> MDE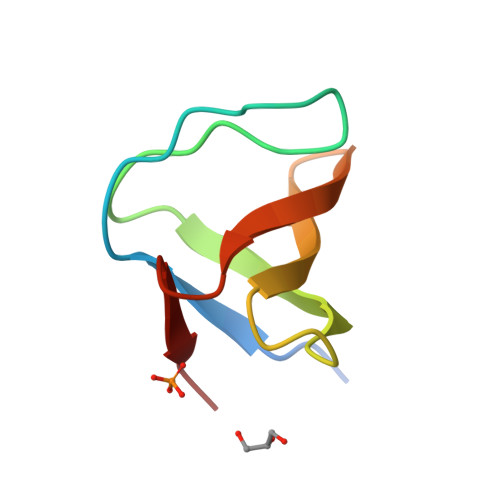TGKELLLVLYDYQEKSPRELTVKKGDILTLLNSTNKDWWKVEWNDRQGFLPAAYLKKLD>[4x]SNAENSEVIKDLYEYLCNVRVHKSYEDDSGL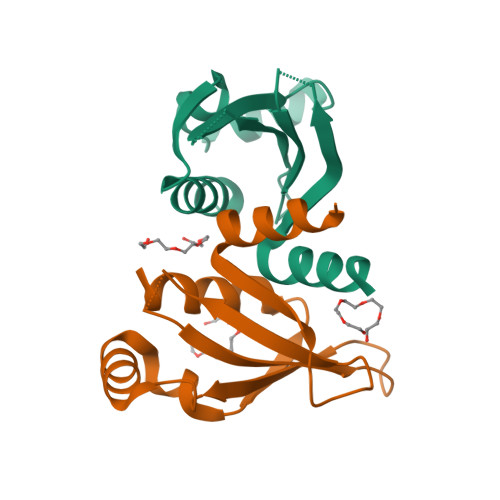WFDISQGTHSGGSSDDYSIMDYKLGFVKGQAQVTEVIYAPVLKQRSTEELYSLQSKLPEYLFETLSFPLSSLNQFYNKIAKSLNK> VDLGSKSSNSTCRLNVTELASIHPGETWTLHGMCISICYYENVTEDEIIGVAFTWQHNESVVDLW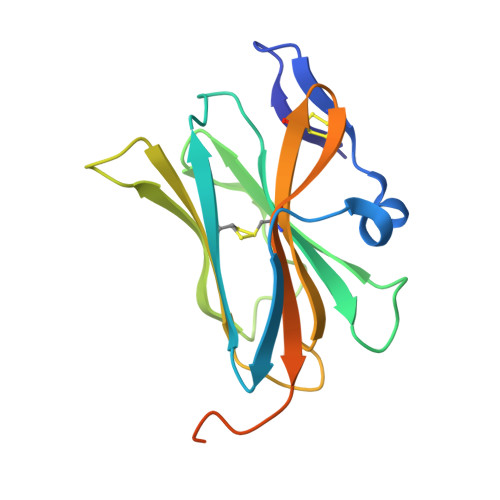LYQNDTVIRNFSDITTNILQDGLKMRTVPVTKLYTSRMVTNLTVGRYDCLRCENGTTKIIERLYVRLGSLYPRPPGSGLAKHPSVSADEELSA> MA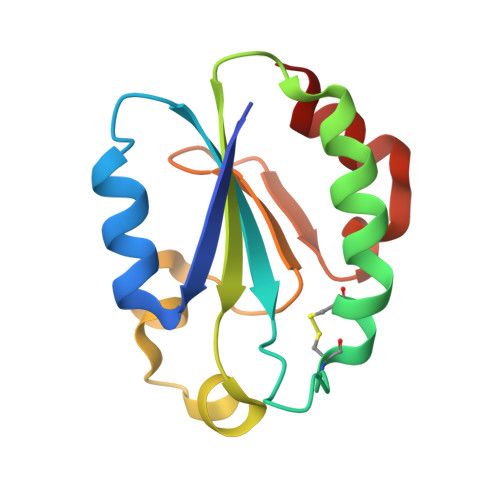RYEEVSVSGFEEFHRAVEQHNGKTIFAYFTGSKDAGGKSWCPDCVQAEPVVREGLKHISEGCVFIYCQVGEKPYWKDPNNDFRKNLKVTAVPTLLKYGTPQKLVESECLQANLVEMLFSED(4~{S},6~{S})-4,6-dimethyloctanoic acid | 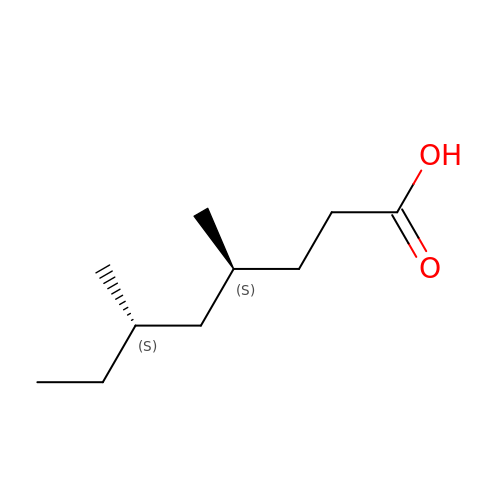C10 H20 O2 | LMFRDZYWEWGVPW-IUCAKERBSA-N[(2~{R},3~{S},4~{R},5~{R})-5-[3-methyl-2,4-bis(oxidanylidene)pyrimidin-1-yl]-3,4-bis(oxidanyl)oxolan-2-yl]methyl 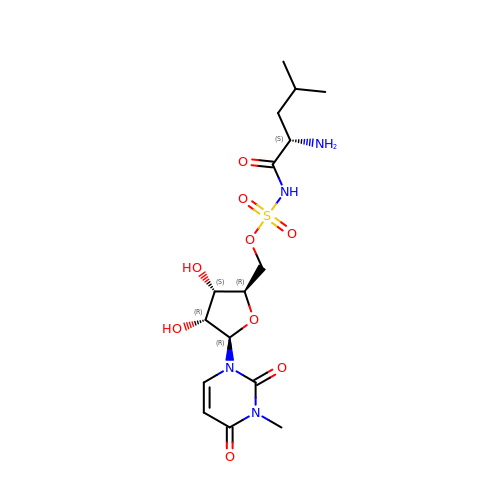~{N}-[(2~{S})-2-azanyl-4-methyl-pentanoyl]sulfamate | C16 H26 N4 O9 S | IHQCOGYAMSEDBL-KHBBOIOASA-N4-ethynyl-N-[(1S,2R)-2-hydroxy-1-(oxocarbamoyl)propyl]benzamide 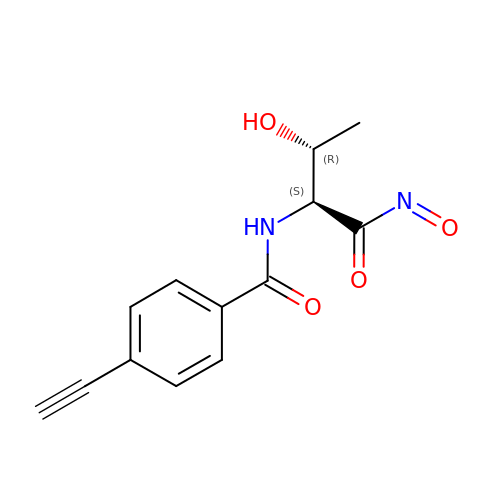| C13 H12 N2 O4 | JJXZDQZGPLQGCP-KCJUWKMLSA-N> IVGGQECKDGECPWQALLINEENEGFCGGTILSEFYILTAAHCLYQAKRFKVRVGDRNTEQEEGGEAVHEVEVVIKHNRFTKETYDFDIAVLRLKTPITFRMNVAPACLPERDWAESTLMTQKTGIVSGFGRTHEKGRQSTRLKMLEVPYVDRNSCKLSSSFIITQN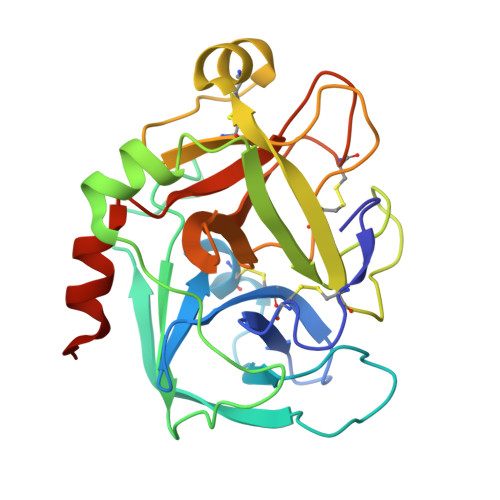MFCAGYDTKQEDACQGDSGGPHVTRFKDTYFVTGIVSWGEGCARKGKYGIYTKVTAFLKWIDRSMKTRGLPKAK>[4x]MSRRNPCKFEIRGHCLNGKRCHFSHNYFEWPPHALLVRQNFMLNRILKSMDKSIDTLSEISGAAELDRTEEYALGVVGVLESYIGSINNITKQSACVAM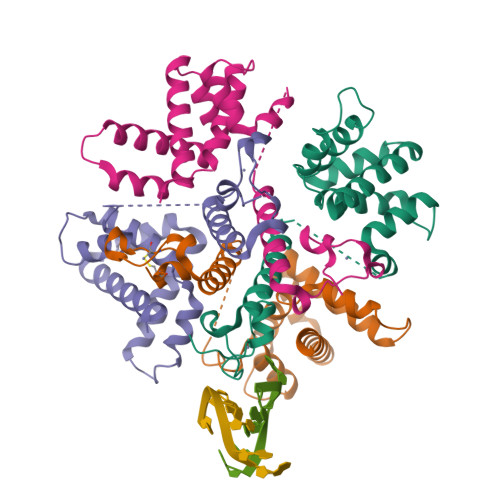SKLLTELNSDDIKKLRDNEELNSPKIRVYNTVISYIESNRKNNKQTIHLLKRLPADVLKKTIKNTLDIHKSITINNPKELTVSDTNDHAKNNDTT>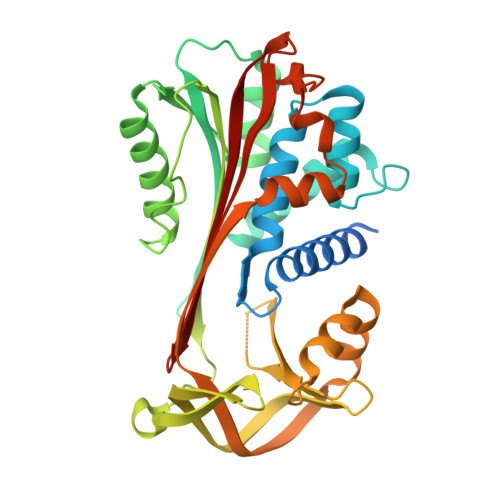 MKHHHHHHMKQNSPLDEENLTQENQDRGTHVDRGLASANVDFAFSLYKQLVLKAPDKNVIFSPVSISTALAFLSLGAHNTTLTEILKGLKFNLTETSEAEIHQSFQHLLRTLNQSSDELQLSMGNAMFVKEQLSLLDRFTEDAKRLYGSEAFATDFQDSAAAKKLINDYVKNGTRGKITDLIKDLDSQTMMVLVNYIFFKAKFEMPFDPQDTHQSRFYLSKKKYVMVPMMSLHHLTIPYFRDEELSCTVVQLNYTGNASALFILPDQDKMEEVEAMLSQETLSRFFESLEFREIGELYLPKFSISRDYNLNDILLQLGIEEAFTSKADLSGITGARNLAVSQVVHKAVLDVFEEGTERSAATALEVLFQ In the heterocystous cyanobacterium Nostoc sp. PCC 7120, one such strategy is the use of an ArsR-SmtB transcriptional regulator RexT that senses H2O2 and upregulates expression of thioredoxin to maintain cellular redox homeostasis. Different from many other members of the ArsR-SmtB family which bind metal ions, RexT has been proposed to use disulfide bond formation as a trigger to bind and release DNA. Here, we present high-resolution crystal structures of RexT in the reduced and H2O2-treated states. These structures reveal that RexT showcases the ArsR-SmtB winged-helix-turn-helix fold and forms a vicinal disulfide bond to orchestrate a response to H2O2. Each protomer of RexT has an α1-α2-α3-α4-β1-β2-α5a/b architecture.

To visualize the structural consequence of Cys residue oxidation, a 2.16-Å resolution structure of H2O2-treated RexT was solved (RexT_Ox). These crystals were prepared by removing crystals of reduced RexT from the anaerobic chamber and immersing them in a solution of cryoprotectant that contained H2O2. The oxidized structure shares a similar overall architecture with that of reduced RexT (rmsd of 0.380 Å for 1258 atoms). In chain A of the RexT dimer, a slight orientation difference is observed for both the Cys40 and Cys41 sidechains relative to the reduced structure. In contrast, in the α3 helix region of chain B, in agreement with the above-described biochemical results, the electron density is consistent with the presence of a disulfide bond between Cys40 and Cys41. To form this disulfide bond, Cys41 undergoes a large conformational change: the sidechain flips −167.8° and moves 8.8-Å away from its position in the reduced structure. Formation of this vicinal disulfide bond results in the creation of an eight-membered ring with the peptide backbone and distortion of the peptide bond geometry. In addition to this observed peptide bond distortion, the movement of Cys41 disrupts the interactions seen in the reduced structure between the backbone and sidechain of Cys41 and residues His75 and Asn77 from the wing of the wHTH motif. The lack of a disulfide bond in chain A is proposed to be due to crystal packing, which would prohibit a comparable movement of these residues. Through this analysis, it was found that a cavity leads from the surface of the protein to a cluster of amino acids that includes Cys41. This cavity contains one molecule of H2O2 in chain A of the H2O2-treated structure and one molecule of glycerol in chain B of the reduced structure, suggesting the possibility that H2O2 gains access to Cys41 using this route. In the oxidized structure, the newly formed disulfide bond is oriented towards the protein surface and perhaps coupled with the architectural changes in RexT, more favorably interacts with reduced TrxA2 and permits subsequent resolving of the disulfide linkage.

>GSMRFLYHPDRKDISLPGVLYALGDPARLEIVRLLASKGEQCCAEFDFAIAKSTMSNHFKILRESGVVLTRKEGTQHINRLRREDLETLFPGLLDAVLRSAQPLLTCQQSAIVK[2x]>GSMTEADVNPKAYPLADAHLTKKLLDLVQQSCNYKQLRKGANEATKTLNRGISEFIVMAADAEPLEIILHLPLLCEDKNVPYVFVRSKQALGRACGVSRPVIACSVTIKEGSQLKQQIQSIQQSIERLLV[2x];>[2x]GPLGSEAAPEYRVIVDANNLTVEIENELNIIHKFIRDKYSKRFPELESLVPNALDYIRTVKELGNSLDKCKNNENLQQILTNATIMVVSVTASTTQGQQLSEEELERLEEACDMALELNASKHRIYEYVESRMSFIAPNLSIIIGASTAAKIMGVAGGLTNLSKMPACNIMLLGAQRKTLSGFSSTSVLPHTGYIYHSDIVQSLPPDLRRKAA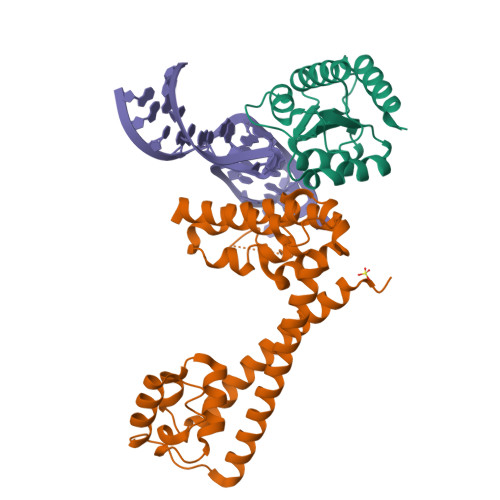RLVAAKCTLAARVDSFHESTEGKVGYELKDEIERKFDKWQE In addition to Alrs, a PLP-dependent racemase is found to possess a broad amino-acid specificity (broad specificity amino acid racemase, Bar, E.C. 5.1.1.10). Notably, Lyr is also active against arginine, whereas Bar racemizes arginine, lysine, methionine, serine, cysteine, leucine, and histidine, a useful feature for biotechnological applications. To further develop lyr- or bar-based marker genes with desired properties, we determined the three-dimensional structures of P. putida DSM84 Bar and P. mirabilis Lyr, which are the first structures for lysine-preferred racemases. All structures contain PLP, which confirms their PLP-dependent nature, and the positions of their catalytic lysines and tyrosines are similar to those in Alr structures.

In addition, the first liganded Bar-lysine structure was also established. The complex-Bar structure was established by co-crystallizing Bar with L-lysine. The final Bar-L-lysine structure had R values of 17.5% (Rfree = 21.9%). The apo and liganded Bar structures share the same two-domain architecture and are both composed of the AB-type dimer. Superposition of the apo- and complex-form reveals a RMSD of 0.34 Å for the Cα atoms, demonstrating an overall identical conformation. The determined Bar-Lys complex structure also shows that the positive guanidium group of Arg261 (corresponding to Arg260 of Lyr) is close to the pyridine nitrogen atom of PLP, hence may not favor the formation of the quinonoid intermediate proposed in the classical two-base mechanism. Moreover, the carboxylate group of L-lysine is situated at a position, allowing hydrogen-bonding interactions with both catalytic bases, respectively. Moreover, structural comparison of complex-Bar structure and Bar-PLY docking model shows that the reactive intermediates (PLP-lysine) are situated at the comparable position and surrounded by identical residues to form resembling hydrogen-bonding networks, suggesting the feasibility of the docking approach utilized here. In conclusion, the determined structures of apo and L-Lys-liganded Bar present the internal and external aldimine linkages, respectively, as well as the anchored substrate in Bar.

>MPFRRTLLAASLALLITGQAPLYAAPPLSMDNGTNALTVQNSNAWVEVSASALQHNIRTLQAELAGKSRLCAVLKADAYGHGIGLVMPSIIAQGVPCVAVASNEEARVVRASGFTGQLVRVRLASLSELEDALQYDMEELVGSAEFARQVDAIAARHGKTLRIHMALNSSGMSRNGVEMATWSGRGEALQITDQKHLKLVALMTHFAVEDKDDVRKGLAAFNEQTDWLIKHAKLDRSKLTLHAANSFATLEVPEARLDMVRTGGALFGDTVPARTEYQRAMQFKSHVAAVHSYPAGNTVGYDRTFTLARDSRLANITVGYSDGYRRVFTNKGHVLINGHRIPVVGKVSMNTLMVDVTDFPDVKGGNEVVLFGKQAGGEITQAEMEEINGALLADLYTVWGSSNPKILVD[2x]>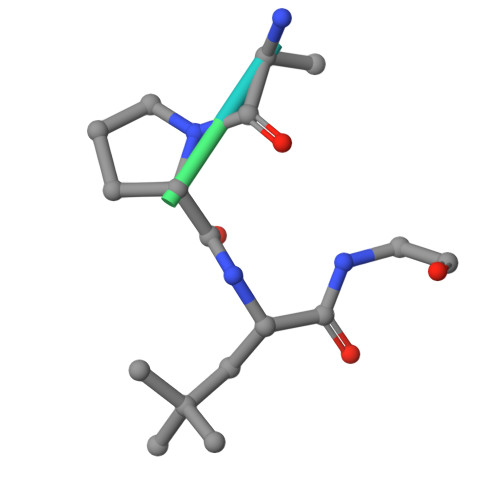 RAPXGDISN> RKPSFLALPGHLVKSEETVILQCWSDVMFEHFLLHREGKFNNTLHLIGEHHDG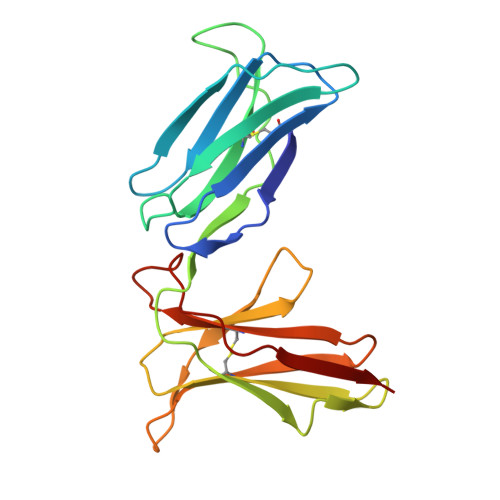VSKANFSIGPMMPVLAGTYRCYGSVPHSPYQLSAPSDPLDMVIIGLYEKPSLSAQPGPTVQAGENVTLSCSSRSSYDMYHLSREGEAHERRLPAVRSINGTFQADFPLGPATHGGTYRCFGSFRDAPYEWSNSSDPLLVSVT We chose TtgR, a ligand-inducible aTF belonging to the diverse TetR-like protein family, as a target for computational engineering of ligand specificity. TtgR is a 1-component transcriptional system and represents the simplest molecular mechanism for converting biophysical interaction between inducer and protein into a complex biological response like transcription. When induced, ligand-binding allosterically lowers affinity for DNA, thereby allowing transcription. TtgR is a compact, dimeric, all-helical transcription factor with a large cavity between five angled helices forming the ligand-binding pocket.

The crystal structure of the computationally designed mutant shows that one of the mutations reshapes the binding pocket to favor resveratrol over naringenin through a striking change in its binding orientation while maintaining allostery. I141W, a mutation critical for resveratrol specificity, creates a large steric barrier that alters the shape of the pocket and obstructs the vertical binding orientation of ligands. Resveratrol is accommodated in the binding pocket in a horizontal binding orientation almost parallel to the plane of the tryptophan. Unlike I141W which plays a clear steric role, the other three mutations (C137I, M167L and F168Y) have a more subtle effect in reshaping the binding pocket through nonpolar interactions. C137I mutation creates a protrusion in the binding pocket that increases shape complementarity to resveratrol. M167L is buried between the residues in the binding pocket and the dimerization helix and may play a role in positioning the I141W tryptophan to stabilize its horizontal orientation through van der Waals interactions. F168Y allows the formation of multiple hydrogen bonds with nearby water molecules and may serve to stabilize the structure. A different hydrogen bonding network consisting of D71, R75, and E78 make hydrogen bonds with the resveratrol molecules in chain A and D71, E78, D172, and a nearby water molecule make a hydrogen bond with the single resveratrol molecule in chain B. The DNA-binding domains of the resveratrol-bound quadruple mutant and the resveratrol-bound wild type are extremely similar with an all-atom RMSD of 1.0 Å. The altered binding mode establishes that allostery is robust to major changes in the binding mode in TtgR.

>SMVRRTKEEAQETRAQIIEAAERAFYKRGVARTTLADIAELAGVTRGAIYWHFNNKAELVQALLDSLHETHDHLARASESEDEVDPLGCMRKLLLQVFNELVLDARTRRINEILHHKCEFTDDMCEIRQQRQSAVLDIHKGWTLALANAVRRGQLPGELDAERAAVALYAYVDGLIRRWLLLPDSVDLLGDVEKWVDTGLDMLRLSPALRK[4x]> MKNYFNSPFKGELLSEQVKNPNIRVGRYSYYSGYYHGHSFDECARYLLPDREDVDKLIIGSFCSIGSGASFIMAGNQGHQHDWASSFPFFYMQEEPAFSRALDAFQRAGDTVIGNDVWIGSEAMIMPGIKIGDGAVIGSRSL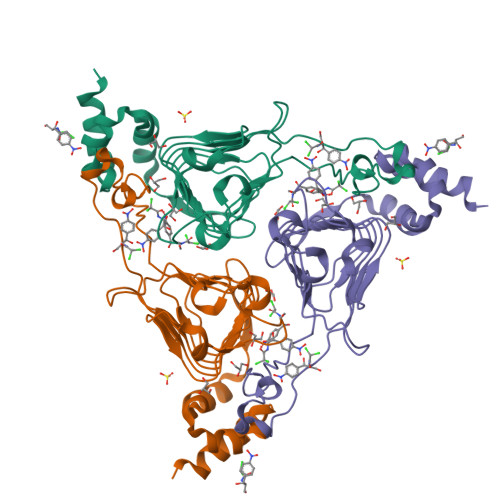VTKDVEPYAIIGGNPAKQIKKRFSDEEISLLMEMEWWNWPLDKIKTAMPLLCSSNIFGLHKYWREFAVLEHHHHHH> AEPFAKLEQDFGGSIGVYAMDTGSGATVSYRAEERFPLCXSFKGFLAAAVLARSQQQAGLLDTPIRYGKNALVPWSPISEKYLTTGMTVAELSAAAVQYSDNAAANLLLKELGGPAGLTAFMRSIGDTTFRLDRWELELNSAIPSDARDTSSPRAVTES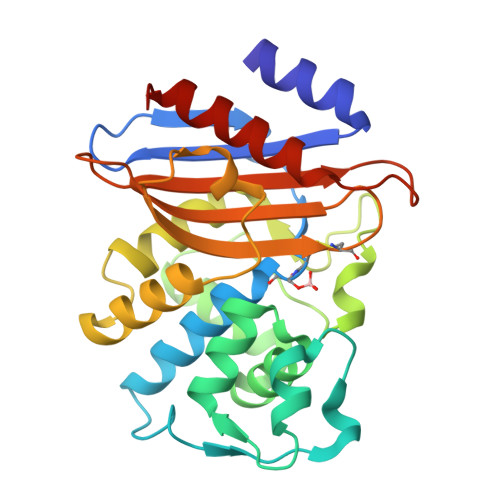LQKLTLGSALAAPQRQQFVDWLKGNTTGNHRIRAAVPADWAVGDKTGTCGVYGTANDYAVVWPTGRAPIVLAVYTRAPNKDDKHSEAVIAAAARLALEGLGVNGQ> MEIKLEEILKKQPL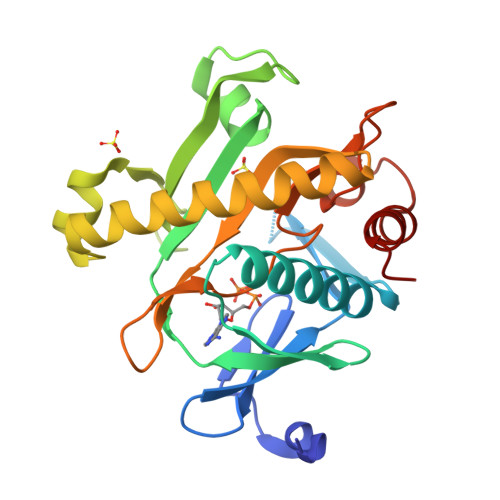YSGKAKSIYEIDDDKVLIEFRDDITAGNGAKHDVKQGKGYLNALISSKLFEALEENGVKTHYIKYIEPRYMIAKKVEIIPIEVIVRNIAAGSLCRRYPFEEGKELPFPIVQFDYKNDEYGDPMLNEDIAVALGLATREELNKIKEIALKVNEVLKKLFDEKGIILVDFKIEIGKDREGNLLVADEISPDTMRLWDKETRDVLDKDVFRKDLGDVIAKYRIVAERLGLL>GHMSRRYWQLDVFAERPLTGNGLAVFDDASALDDAAMQAWTRELRQFESIFLLPGDDPRAFRARIFTLEEELPFAGHPLLGAAALLHHLRG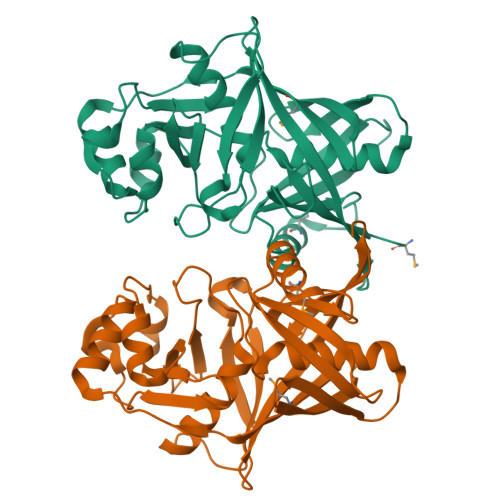GDNEQHWTLHLASKSVALRSVRAGSGFYAEMDQGRAEFGATPDAGTCRWFAEAFSLSANDLSGHPPRVVSTGLPYLLLPVTAEALGRARQVNDLQEALDKLGAAFVYLLDVDGREGRTWDNLGLVEDVATGSAAGPVAAYLVEYGLAARGEPFVLHQGRFLERPSRLDVQVATDGSVRVGGHVQLLARAELLTSAGS[2x]> MSIWKEAKDASGRIYYYNTLTKKSTWEKPKELISQEELLLRENGWKAAKTADGKVYYYNPTTRETSWTIPAFEKKVEPIAEQKHDTVSHAQVNGNRIALTAGEKQEPGRTINEEESQYANNSKLLNVRRRT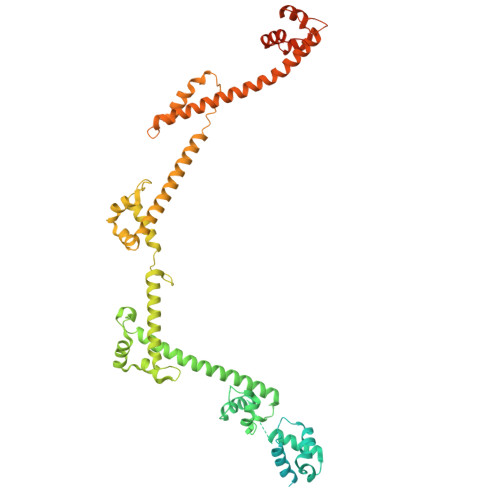KEEAEKEFITMLKENQVDSTWSFSRIISELGTRDPRYWMVDDDPLWKKEMFEKYLSNRSADQLLKEHNETSKFKEAFQKMLQNNSHIKYYTRWPTAKRLIADEPIYKHSVVNEKTKRQTFQDYIDTLIDTQKESKKKLKTQALKELREYLNGIITTSSSETFITWQQLLNHYVFDKSKRYMANRHFKVLTHEDVLNEYLKIVNTIENDLQNKLNELRLRNYTRDRIARDNFKSLLREVPIKIKANTRWSDIYPHIKSDPRFLHMLGRNGSSCLDLFLDFVDEQRMYIFAQRSIAQQTLIDQNFEWNDADSDEITKQNIEKVLENDRKFDKVDKEDISLIVDGLIKQRNEKIQQKLQNERRILEQKKHYFWLLLQRTYTKTGKPKPSTWDLASKELGESLEYKALGDEDNIRRQIFEDFKPESSAPTAESATANLTLTASKKRHLTPAVELDY>MYDWFSEMRKKDPVYYDGNIWQVFSYRYTKEVLNNFSKFSSDLTGYHERLEDLRNGKIRFDIPTRYTMLTSDPPLHDELRSMSADIFSPQKLQTLETFIRETTRSLLDSIDPREDDIVKKLAVPLPIIVISKILGLPIEDKEKFKEWSDLVAFRLGKPGEIFELGKKYLELIGYVKDHLNSGTEVVSRVVNSNLSDIEKLGYIILLLIAG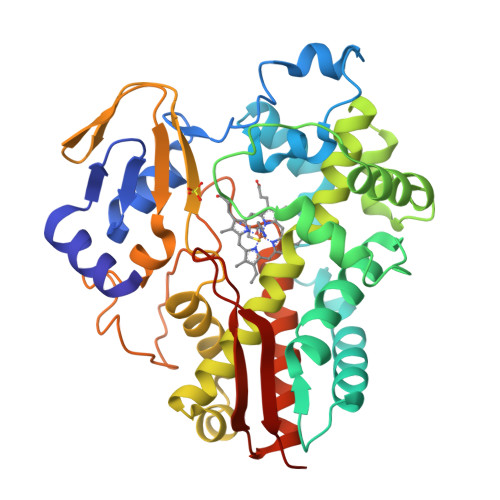NETTTNLISNSVIDFTRFNLWQRIREENLYLKAIEEALRYSPPVMRTVRKTKERVKLGDQTIEEGEYVRVWIASANRDEEVFHDGEKFIPDRNPNPHLSFGSGIHLCLGAPLARLEARIAIEEFSKRFRHIEILDTEKVPNEVLNGYKRLVVRLKSNE[2x]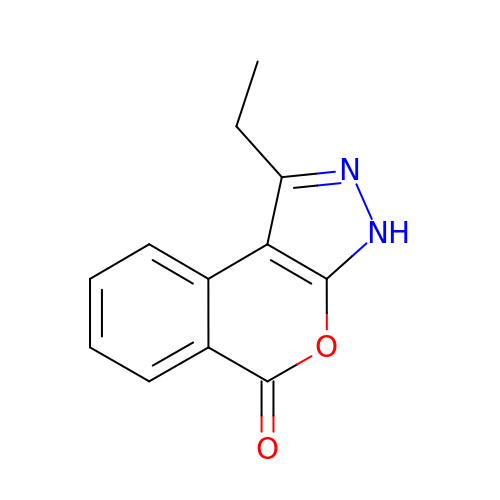1-ethylisochromeno[3,4-c]pyrazol-5(3H)-one | C12 H10 N2 O2 | MKAQORNERCMQLJ-UHFFFAOYSA-N> MAFSVNYDSSFGGYSIHDYLGQWASTFGDVNHTNGNVTDANSGGFYGGSLSGSQYAISSTANQVTAFVAGGNLTYTLFNEPAHTLYGQLDSLSFGDGLSGGDTSPYSIQVPDVSFGGLNLSSLQAQGHDGVVHQVVYGLMSGDTGALETALNGILDD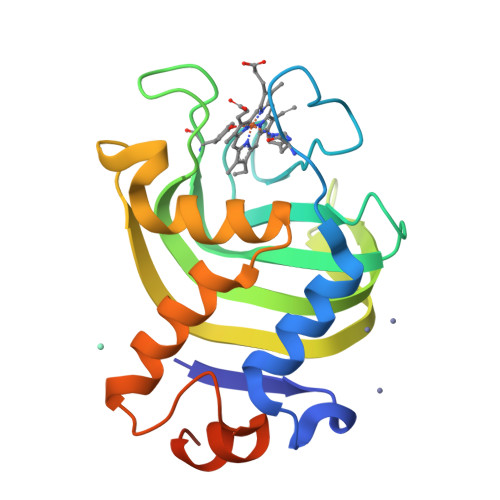YGLSVNSTFDQVAAATAVGVQHADSPELLAA>MTNKISSSDNLSNAVSATDDNASRTPNLNRRALVGGGVGLAARGALASGLQAATLPAGASQVPTTPAGRPMPYAIRPMPEDRRFGYAIVGLGKYALNQILPGFAGCQHSRIEALVSGNAEKAKIVAAEYGVDPRKIYDYSNFDKIAKDPKIDAVYIILPNSLHAEFAIRAFKAGKHVMCEKPMATSVADCQRMIDAAKAANKKLMIGYRCHYDPMNRAAVKLIRENQLGKLGMVTTDNSDVMDQNDPAQQWRLRRELAGGGSLMDIGIYGLNGTRYLLGEEPIEVRAYTYSDPNDERFVEVEDRIIWQMRFR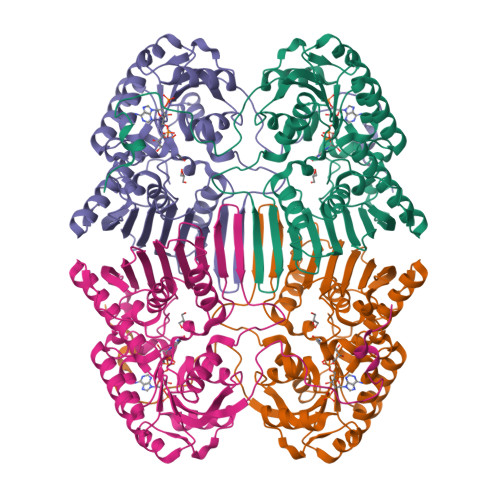SGALSHGASSYSTTTTSRFSVQGDKAVLLMDPATGYYQNLISVQTPGHANQSMMPQFIMPANNQFSAQLDHLAEAVINNKPVRSPGEEGMQDVRLIQAIYEAARTGRPVNTDWGYVRQGGY[2x]> MPLDPVIQQVLDQLNRMPAPDYKHLSAQQFRSQQSLFPPVKKEPVAEVREFDMDLPGRTLKVRMYRPEGVEPPYPALVYYHGGGWVVGDLETHDPVCRVLAKDGRAVVFSVDYRLAPEHKFPAAVEDAYDAL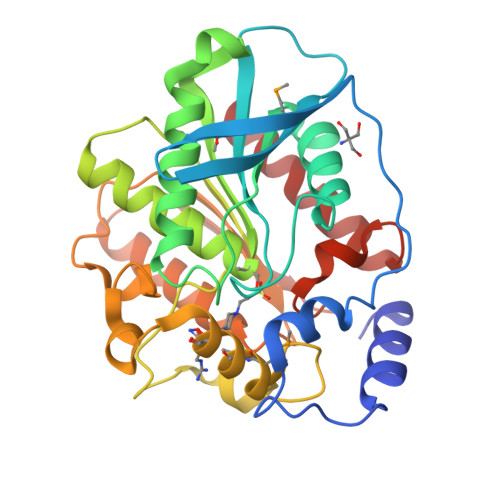QWIAERAADFHLDPARIAVGGDSAGGNLAAVTSILAKERGGPALAFQLLIYPSTGYDPAHPPASIEENAEGYLLTGGMMLWFRDQYLNSLEELTHPWFSPVLYPDLSGLPPAYIATAQYDPLRDVGKLYAEALNKAGVKVEIENFEDLIHGFAQFYSLSPGATKALVRIAEKLRDALA> ETDEEPEEPGRRGSFVEMVDNLRGKSGQGYYVEMTVGSPPQTLNILVDTGSSNFAVGAAPHPFLHRYYQRQLSSTYRDLRKGVYVPYTQGKWEGELGTDLVSIPHGPNVTVRANIAAITESDKFFINGSNWEGILGLAYAEIARPDDSLEPFFDSLVKQTHVPNLFSLQLCGAGFPLNQSEVLASVGGSMIIGGIDHSLYTGSLWYTPIRREWYYEVIIVRVEINGQDLKMDCKEYNYDKSIVDSGTTNLRLPKKVFEAAVKSIKAASSTEKFPDGFWLGEQLVCWQAGTTPWNIFP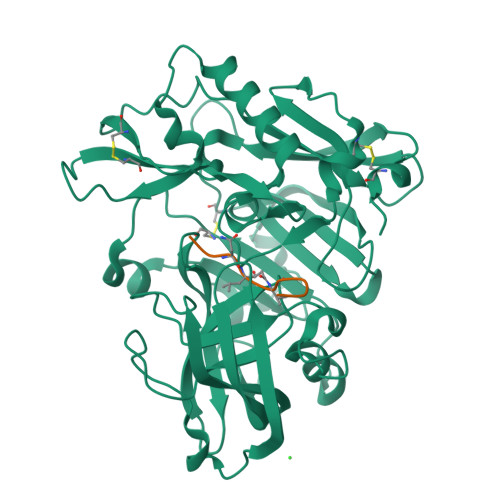VISLYLMGEVTNQSFRITILPQQYLRPVEDVATSQDDCYKFAISQSSTGTVMGAVIMEGFYVVFDRARKRIGFAVSACHVHDEFRTAAVEGPFVTLDMEDCGYNIPQTDEST;> EVNXVAEPKX> GSSRAMGNEVAGVEDISVEITPSSKRNSDARRTSRNCSSNEERKRRKYFHMLYLVCLMVHGFIRNEWINSKRLSRKLSNLVPEKVFELLHPQKDEELPLRSTRKLLDGLKKCMELWQKHWKITKKYDNEGLYMRTWKEIEMSANNKRKFKTLKRSDFLRAVSKGHGDPDISVQGFVAMLRACNVNARLIMSCQPPDFTNMKIDTSLNGNNAYKDMVKYPIFWCEVWDKFSKKWITVDPVNLKTIEQVRLHSKLAPKGVACCERNMLRYVIAYDRKYGCRDVTRRYAQWMNSKVRKRRITKDDFGEKWFRKVITALHHRKRTKIDDYEDQYFFRRDESEGIPDSVQDLKNHPYYVLEQDIKQTQIVKPGCKECGYLKVHGKVGKVLKVYAKRDIADLKSARQWYMNGRILKTGSRCKKVIKRTVGRPKGEAEEEDERLYSFEDTELYIPPLASASGEITKNTFGNIEVFAPTMIPGNCCLVENPVAIKAARFLGVEFAPAVTSFKFERGSTVKPVLSGIVVAKWLREAIETAIDGIEFI;> GSGNASSGALGTTGGATDAAQGGPPGSIGLTVEDLLSLRQVVSGNPEALAPLLENISARYPQLREHIMANPEVFVSMLLEAVGDNMQDVMEGADDMVEGEDIEVTGEAAAAGLGQGEGEGSFQVDYTPEDDQAISRLCELGFER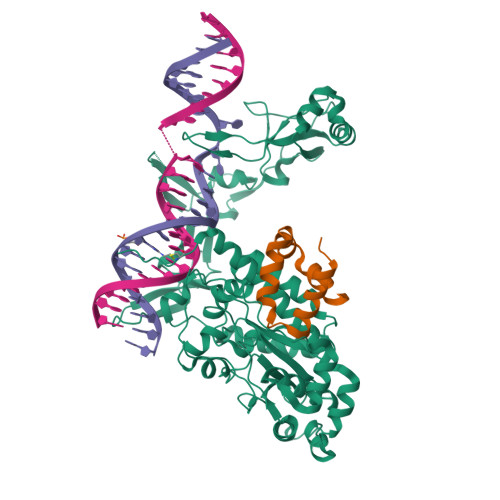DLVIQVYFACDKNEEAAANILFSDHAD>[4x]SMTIRFHRNDLPNLDNYQVDAVAIDTETLGLNPHRDRLCVVQISPGDGTADVIQIEAGQKKAPNLVKLLKDRSITKIFH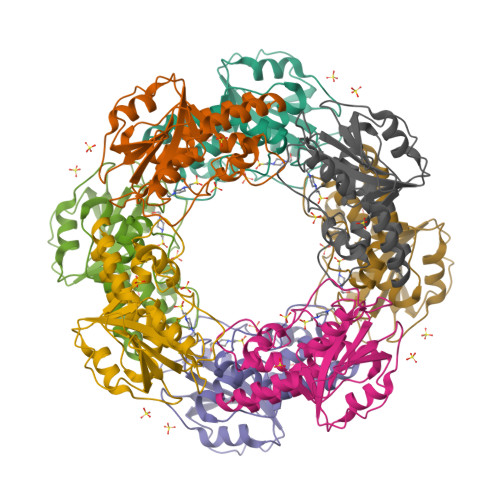FGRFDLAVLAHAFGTMPQPVFCTKIASKLTRTYTDRHGLKEICSELLDVSISKQQQSSDWAAEVLSQAQLEYAASDVLYLHRLKAVLEQRLERDGRTKQAEACFKFLPTRSELDLMGWAESDIFAHS>[2x]MKDWLFRIATCSIMTFSSLAAAQAEPLDVVATFSIIGDFAAKVGGDRIRLNVLVGPDSDTHVYEPRPADAIALAGADVVLT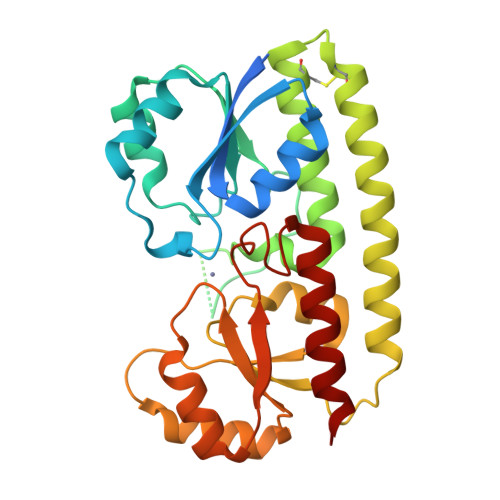NGLEFEGFLTRLIAASGTDAAVATLTDGVETMEEPGGGHYHYIDGKAVFHAGAHDPHAWQAVPNAKVYVQNIAAAFCAADAEGCAAYQANAARYIGELDALDTEIRAAIAALPQDRRTVVVAHNAFRYFEAAYGVHFLSPAAAADVAGLIREIRARNASAIFAENISDTRLLEQIAREAGLPLAGTLYSDALSGPDGPASNYIAMMRHNAGAIAAALAAR>SNAMSTIARRGFHYMQRLNSANVSPALLEKAQNRVIDAALTFIRERAKFKGELMRSLGGVAATSSLLGVPLGHHSSFHEGSAFAPPRIREAIWCDSTNSTTEEGKNLRDPRVITNVGDVPIEEIRDCGVDDKRLANVISESVKLVMDEDPLRPLVLGGDHSISFPVVRAVSEKLGGAVDILHFDAHPDLYHDFEGNYYSHASPFARIMEGGYARRLVQVGIRSITNDVREQVKKYGVETHEMRTLSRDRPILENLKLGEGVKGVYVSIDVDS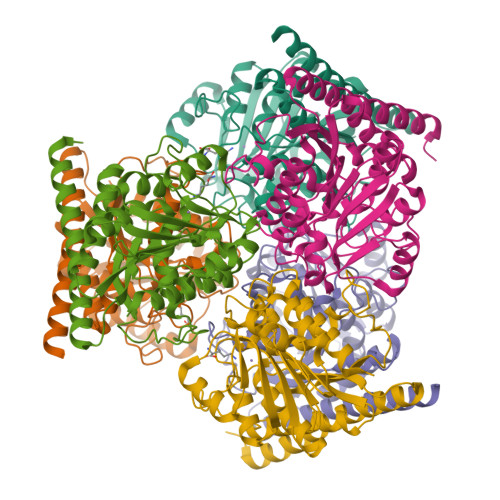LDPSIAPGVSHHEPGGLLFRDILNILQNLQGDIVGGDVVEYNPQRDTYDGITALVAAKLVRELAAKMSK[12x]>GPHMLEHSGISQASEYDDPPGLREKAEYLLREWVNLYHSAAAGRDSTKAFSAFVGQMHQQGILKTDDLITRFFRLCTEMCVEISYRAQAEQQHNPAANPTMIRAKCYHNLDAFVRLIALLVKHSGEATNTVTKINLLNKVLGIVVGVLLQDHDVRQSEFQQLPYHRIFIMLLLELNAPEHVLETINFQTLTAFCNTFHILRPTKAPGFVYAWLELISHRIFIARMLAHTPQQKGWPMYAQLLIDLFKYLAPFLRNVELTKPMQILYKGTLRVLLVLLHDFPEFLCDYHYGFCDVIPPNCIQLRNLILSAFPRNMRLPDPFTPNLKVDMLSEINIAPRILTNFTGVMPPQFKKDLDSYLKTRSPVTFLSDLRSNLQVSNEPGNRYNLQLINALVLYVGTQAIAHIHNKGSTPSMSTITHSAHMDIFQNLAVDLDTEGRYLFLNAIANQLRYPNSHTHYFSCTMLYLFAEANTEAIQEQITRVLLERLIVNRPHPWGLLITFIELIKNPAFKFWNHEFVEEEPEIEKLFQSVAQCCM[2x];>[2x]GPHMLEMVTDQFGMIGLLTFIRAAETDPGMVHLALGSDLTTLGLNLNSPENLYPKFASPWASSPCRPQDIDFHVPSEYLTNIHIRDKLAAIKLGRYGEDLLFYLYYMNGGDVLQLLAAVELFNRDWRYHKEERVWITRAPGMEPTMKTNTYERGTYYFFDCLNWRKVAKEFHLEYDKLEERPHLPSTFNYNPAQQAF;>[2x]GPHMLELTKEQLYQQAMEEAAWHHMPHPSDSERIRQYLPRNPCPTPPYHHQMPPPHSDTVEFYQRLSTETLFFIFYYLEGTKAQYLA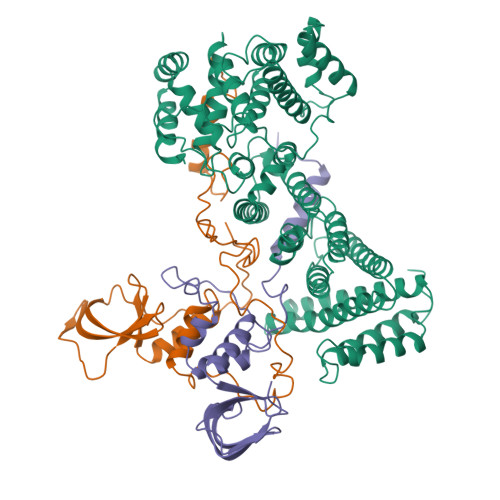AKALKKQSWRFHTKYMMWFQRHEEPKTITDEFEQGTYIYFDYEKWGQRKKEGFTFEYRYLE>MKKTKIVCTIGPKTESEEMLAKMLDAGMNVMRLNFSHGDYAEHGQRIQNLRNVMSKTGKTA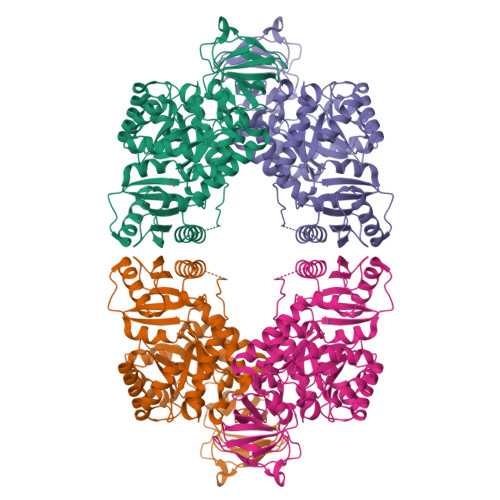AILLDTKGPEIRTMKLEGGNDVSLKAGQTFTFTTDKSVIGNSEMVAVTYEGFTTDLSVGNTVLVDDGLIGMEVTAIEGNKVICKVLNNGDLGENKGVNLPGVSIALPALAEKDKQDLIFGCEQGVDFVAASFIRKRSDVIEIREHLKAHGGENIHIISKIENQEGLNNFDEILEASDGIMVARGDLGVEIPVEEVIFAQKMMIEKCIRARKVVITATQMLDSMIKNPRPTRAEAGDVANAILDGTDAVMLSGESAKGKYPLEAVSIMATICERTDRVMNSRLEFNNDNRKLRITEAVCRGAVETAEKLDAPLIVVATQGAKSARAVRKYFPDATILALTTNEKTAHQLVLSKGVVPQLVKEITSTDDFYRLGKELALQSGLAHKGDVVVMVSGALVPSGTTNTASVHVL[2x]>[2x]MGSDKIHHHHHHENLYFQGMMKFFEYNWQVRDQWFTWCHQLTTEELLKNRLGGVENILYTLFHIIDVEYSWIRAIQGKEDIAVQFADYQTLNKVKSLSNTFRTEIIDVLQTHSDQIKDE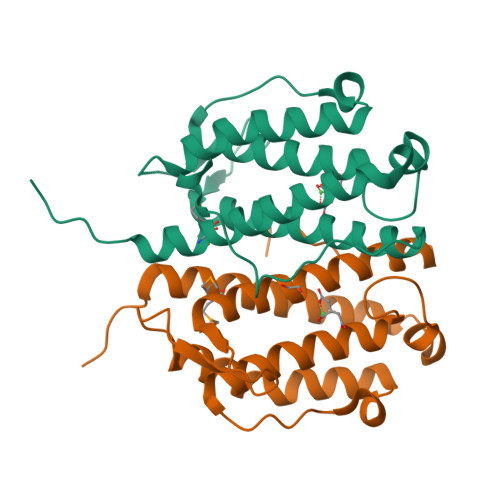LVSVPWETGVLYTRDEILHHIIAHEIHHIGQLSVWARELKLSPVSASFIGRTLKPIHSY> MEDKGKTFFGQPLGLSTLFMTEMWERFSYYGMRAILLYYMWFLISTGDLHITRATAASIMAIYASMVYLSGTIGGFVADRIIGARPAVFWGGVLIMLGHIVLALPFGASALFGSIILIIIGTGFLKPNVSTLVGTLYDEHDRRRDAGFSIFVFGINLGAFIAPLIVGAAQEAAGYHVAFSLAAIGMFIGLLVYYFGGKKTLDPHYLRPTDPLAPEEVKPLLVKVSLAVAGFIAIIVVMNLVGWNSL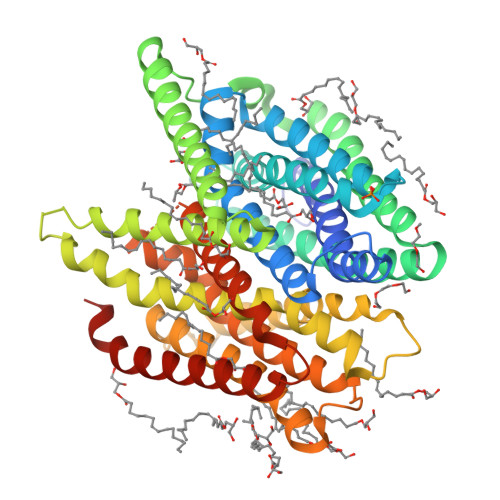PAYINLLTIVAIAIPVFYFAWMISSVKVTSTEHLRVVSYIPLFIAAVLFWAIEEQGSVVLATFAAERVDSSWFPVSWFQSLNPLFIMLYTPFFAWLWTAWKKNQPSSPTKFAVGLMFAGLSFLLMAIPGALYGTSGKVSPLWLVGSWALVILGEMLISPVGLSVTTKLAPKAFNSQMMSMWFLSSSVGSALNAQLVTLYNAKSEVAYFSYFGLGSVVLGIVLVFLSKRIQGLMQGVE8-HYDROXY-2-OXA-BICYCLO[3.3.1]NON-6-ENE-3,5-DICARBOXYLIC 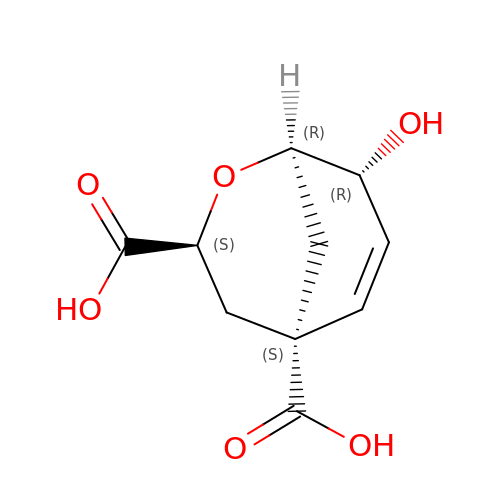ACID | C10 H12 O6 | KRZHNRULRHECRF-JQCUSGDOSA-N>[2x]EWSHPQFEKGGQETSINCKNIQSTQLTIEHLSKCMAFYQ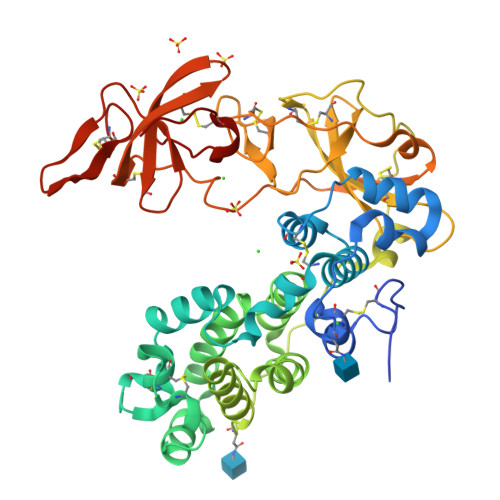NKTSSPVVINEIISDASVDEQELIKSLNLNCNVIDRFISESSVIETQVYYEYIKSQLCPLQVHDIFTINSASNIQWKALARSFTLGVCNTNPHKHICRCLESMQMCTSTKTDHAREMSIYYDGHPDRFEHDMKIILNIMRYIVPGLGRVLLDQIKQTKDYQALRHIQGKLSPKSQSNLQLKGFLEFVDFILGANVTIEKTPQTLTTLSLIKGAHRNLDQKDPGPTPILVCKSPQKVVCYSPRGVTHPGDYISCKSKMYKWPSLGVYKHNRDQQQACSSDTHCLEMFEPAERTITTKICKVSDMTYSESPYSTGIPSCNVKRFGSCNVRGHQWQIAECSNGLFYYVSAKAHSKTNDITLYCLSANCLDLRYAFRSSSCSDIVW We have been interested in a D-aminoacyl-tRNA deacylase (DTD) fold that is present across the domains of life in two different functional contexts: as an N-terminal editing domain (NTD) of archaeal ThrRS, which specifically removes non-cognate L-serine mischarged on tRNAThr, and as a freestanding ‘chiral proofreading' enzyme, which removes D-amino acids from tRNAs in bacteria and eukaryotes. Both share a striking structural and mechanistic similarity highlighting a common ancestry. Here we show, with the help of structural, biochemical and biophysical studies from three distant organisms, that the substrate specificity in this domain is determined by a differential remodelling of the catalytic centre at the RNA–protein interface rather than just the presence or absence of catalytic water as previously proposed. While demonstrating that the tRNA provides the catalytic group, we show that the side chains within the recognition site are dispensable for the proofreading function, suggesting a primordial mode of protein- or peptide scaffold-based enzymatic activity evolved alongside that of RNA.

To understand this intriguing mechanism of cognate substrate rejection in NTD, we have solved high-resolution crystal structures of ApNTD, as well as NTD from Methanococcus jannaschii (MjNTD) in complex with non-cognate and cognate substrate analogues L-seryl-3′-aminoadenosine (L-Ser3AA) and L-threonyl-3′-aminoadenosine (L-Thr3AA), respectively. In the case of MjNTD, L-Ser3AA and L-Thr3AA complex were crystallized in C2 and P21 space groups with six and four monomers, respectively, in the asymmetric unit corresponding to three and two dimers. However, a clear and complete ligand density was observed in only chain A in the case of MjNTD co-crystals and therefore only this monomer was used for analysis. The possible reason for this could be the remarkably low binding affinity for the ligand in MjNTD, as revealed by binding studies later in this section. Second, and more importantly, just the presence or absence of the water Wat1 is not sufficient to determine whether the substrate would be deacylated by the enzyme or not, since Wat1 is also present in the MjNTD+L-Thr3AA structure. There was a clear activity against L-Ser-(Ec)tRNAThr while no deacylation was observed against L-Thr-(Ec)tRNAThr even though Wat1 was present in both L-Ser3AA- and L-Thr3AA-bound structures. The lack of activity against L-Thr-(Ec)tRNAThr by MjNTD strongly suggests a role of other determinants besides the presence/absence of Wat1 in substrate discrimination. On the other hand, in ApNTD and MjNTD it leads to a loosening of interactions of the threonyl moiety of the substrate in the pocket, which would not allow it to be fixed with sufficient rigidity for the nucleophilic attack to take place. While this loosening of interactions is very striking in the case of MjNTD, in ApNTD there is a subtle relaxation.

>MKMLLIHSDYLEFEAKEKTKIAEETENLKGKLDECLACFIAVEREDENNPEGTAIGAVEEIEKVANQLKVNNIVVYPYAHLSSDLSSPETAVKVLKDIESILKERGYNVLRAPFGWYKAFKISCKGHPLSELSRKIVAKEE[4x]> MSLFGTTSGFGTSGTSMFGSATTDNHNPMKDIEVTSSP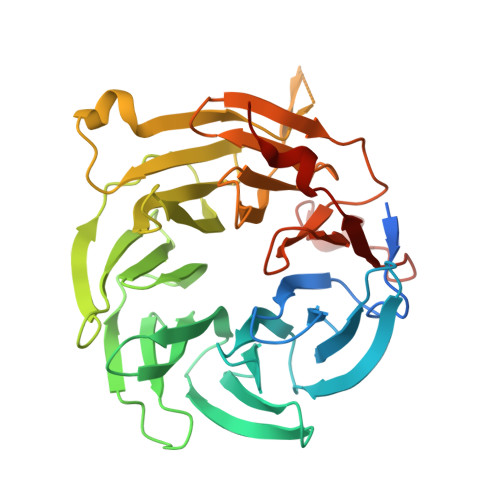DDSIGCLSFSPPTLPGNFLIAGSWANDVRCWEVQDSGQTIPKAQQMHTGPVLDVCWSDDGSKVFTASCDKTAKMWDLSSNQAIQIAQHDAPVKTIHWIKAPNYSCVMTGSWDKTLKFWDTRSSNPMMVLQLPERCYCADVIYPMAVVATAERGLIVYQLENQPSEFRRIESPLKHQHRCVAIFKDKQNKPTGFALGSIEGRVAIHYINPPNPAKDNFTFKCHRSNGTNTSAPQDIYAVNGIAFHPVHGTLATVGSDGRFSFWDKDARTKLKTSEQLDQPISACCFNHNGNIFAYASSYDWSKGHEFYNPQKKNYIFLRNAAEELKPRNKK>MVAPAGEQGRSSTALSDNPFDAKAWRLVDGFDDLTDITYHRHVDDATVRVAFNRPEVRNAFRPHTVDELYRVLDHARMSPDVGVVLLTGNGPSPKDGGWAFCSGGDQRIRGRSGYQYASGDTADTVDVARAGRLHILEVQRLIRFMPKVVICLVNGWAAGGGHSLHVVCDLTLASREYARFKQTDADVGSFDGGYGSAYLARQVGQKFAREIFFLGRTYTAEQMHQMGAVNAVAEHAELETVGLQWAAEINAKSPQAQRMLKFAFNLLDD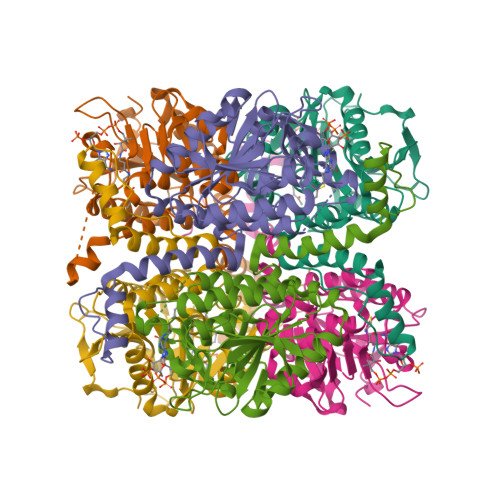GLVGQQLFAGEATRLAYMTDEAVEGRDAFLQKRPPDWSPFPRYF[12x]>[2x]GPGIAVSDDCVQKFNELKLGKKHRYVIFKLNDDNTEVVVEKVGGPNATYEDFLAQLPENDCRYAIFDYEFEVDGGQRNKI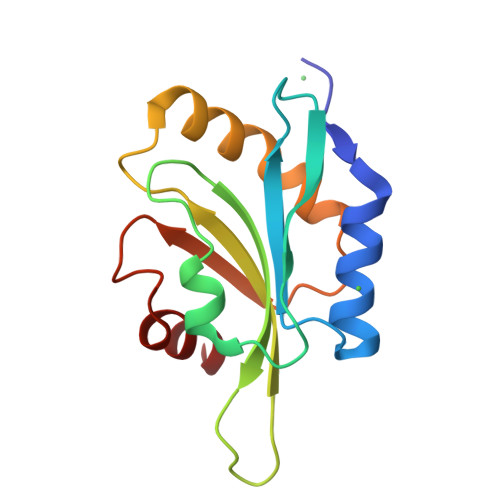VFILWAPDSAPIKSKMMYASSKDAIKKKLDGIQVEVQATDADEISEDAVKERAKK2-({6-[(3-CHLOROPHENYL)AMINO]-9-ISOPROPYL-9H-PURIN-2-YL}AMINO)-3-METHYLBUTAN-1-OL | C19 H25 Cl N6 O | 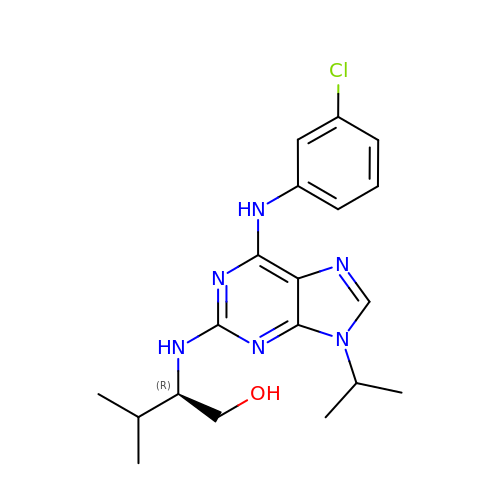PMXCMJLOPOFPBT-HNNXBMFYSA-N> SNAMSEQSICQARAAVMVYDDANKKWVPAGGSTGFSRVHIYHHTGNN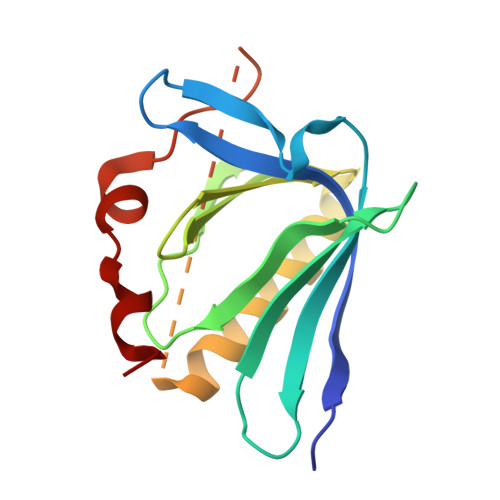TFRVVGRKIQDHQVVINCAIPKGLKYNQATQTFHQWRDARQVYGLNFGSKEDANVFASAMMHALEVLGGSGSGAAKSEELSCEMEGNLEHLPPPPMEVLMDKSFASLES> PIQQLPMMKGMGKDFKNADYIDYLPVNMLATPKEILNSSGYLRSFPGITKRYDMNGVSRGVEYNTAQNAVYRVCGGKLYKGESEVGDVAGSGRVSMAHGRTSQAVGVNGQLVEYRYDGTVKTVSNWPADSGFTQYELGSVRDITRLRGRYAWSKDGTDSWFITDLEDESHPDRYSAQYRAESQPDGIIGIGTWRDFIVCFGSSTIEYFSLTGATTAGAALYVAQPSLMVQKSIAGTYCKT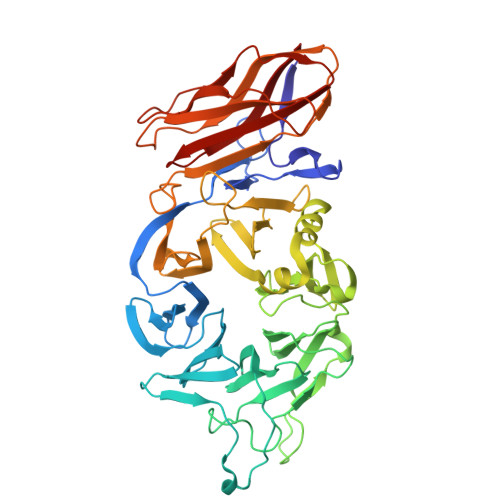PFADSYAFISHPATGAPSVYIIGSGQASPIATASIEKIIRSYTAEEMATGVMETLRFDSHELLIIHLPRHVLVYDASSSQNGPQWCVLKTGLYDDVYRGVDFMYEGNQITCGDKSEAVVGQLQFDISSQYDKQQEHLLFTPLFKADNARCFDLEVESSTGVAQYADRLFLSATTDGINYGREQMIEQNEPFVYDKRVLWKRVGRIRRLIGFKLRVITKSPVTLSGCQIRLE> GHMEPAAS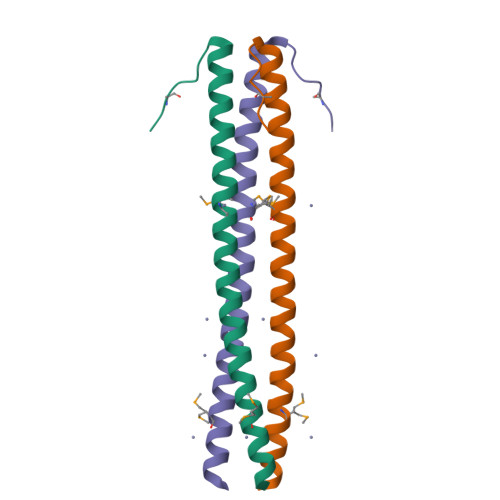SQAAVEELRTQVRELRSIIETMKDQQKREIKQLLSELDEEKKIRLRLQMEVNDIKKAL>MHHHHHHTSKIEQPRWASKDSAAGAASTPDEKIVLEFVDALTSNDAAKLIEYFAEDTMYQNMPLPPAYGRDAVEQTLAGLFTVVSVDAVETFHIGSSNGLVYTERVDVLR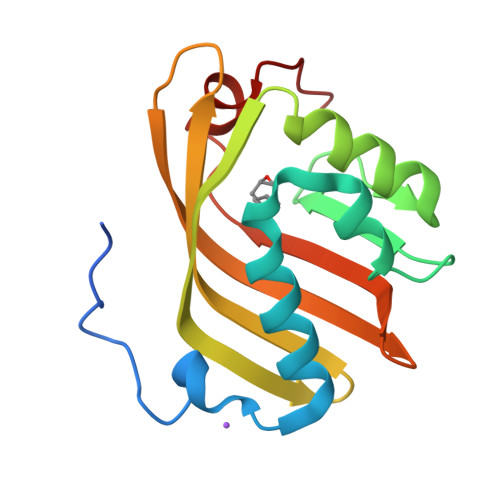ALPTGKSYNFSILGVFQLTEGKITGWRDYFDLREFEEAVDLPLRG[2x]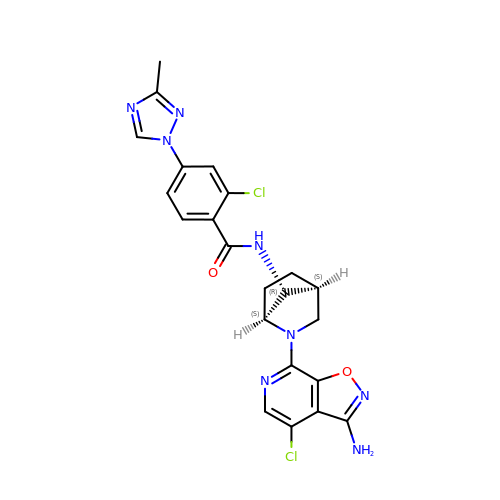N-[(1S,4S,7R)-2-(3-amino-4-chloro[1,2]oxazolo[5,4-c]pyridin-7-yl)-2-azabicyclo[2.2.1]heptan-7-yl]-2-chloro-4-(3-methyl-1H-1,2,4-triazol-1-yl)benzamide | C22 H20 Cl2 N8 O2 | KWAYYBDVPSPGPN-SDDDUWNISA-N>[5x]DLLSWFKGNDRPPAPAGKALEFSKPAAWQNNLPLTPADKVSGYNNFYEFGLDKADPAANAGSLKTDPWTLKISGEVAKPLTLDHDDLTRRFPLEERIYRMRCVEAWSMVVPWIGFPLHKLLALAEPTSNAKYVAFETIYAPEQMPGQQDRFIGGGLKYPYVEGLRLDEAMHPLTLMTVGVYGKALPPQ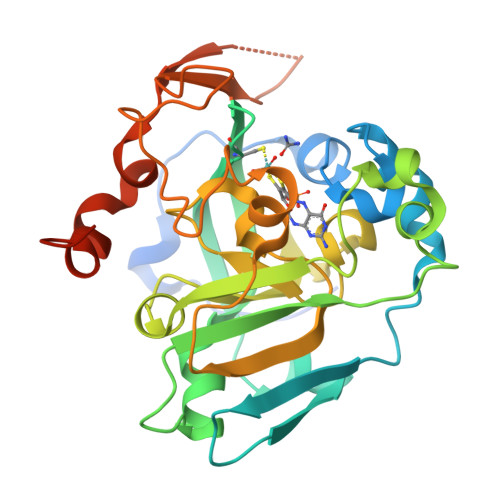NGAPVRLIVPWKYGFKGIKSIVSIKLTRERPPTTWNLAAPDEYGFYANVNPYVDHPRWSQATERFIGSGGILDVQRQPTLLFNGYADQVASLYRGLDLRENFLEHHHHHH>GSHMASMTGGQQMGRGSMKFSFELAVNTKKEDAWTYYSQVNQWFVWEGDLEQISLEGEFTTGQKGKMKMEDMPELAFTLVEVRENQCFSDLTATPFGNVLFEHEILENPDGTISLRHSVSLTDSDTTEEALAFLKQIFADVPESVGKLKQILETV[2x]

One such case is SMU.440 (GeneID: 1029579), which is composed of 138 residues. SMU.440 is a hypothetical protein without any known functions or protein family classification. The crystal structure reveals a fold similar to known polyketide cyclases even though the amino acid sequences are quite different. SMU.440 also shares a similar binding pocket composed primarily of residues with aromatic and acidic side-chains, which points to a potential binding of a polyketide-like molecule.

The crystal structure of SMU.440 has been determined at 2.4 Å resolution using the SIRAS (single isomorphous replacement with anomalous scattering) method and all residues except the last one could be fitted into the electron density. In addition, five residues from the N-terminal His6-tag were also observed in the structure. SMU.440 is comprised of three α-helices and a seven-stranded antiparallel β-sheet, bending into an unclosed β-barrel. The structure belongs to the SCOP superfamily of Bet v1-like proteins. There are two molecules per asymmetric unit (ASU) and they form a homodimer via a pair of antiparallel β-strands. Prediction of assemblies by the PISA server indicates that this dimer interface is the largest (interface area 946.6 Å2) with a favorable interaction energy (ΔiG −6.9 kcal/mol), in agreement with the dimer state in solution observed during the gel filtration chromatography experiment. A large forked cavity is formed as the β-barrel wraps around the long C-terminal α3-helix. The volume of the cavity is about 1 050 Å3 with a surface area of ∼700 Å2. The cavity is comprised of Trp26, Trp29, Glu30, Asp32, Met50, Met52, Met55, Phe60, Phe71, Asp73, Thr75, Thr77, Val82, Phe84, His86, His100, Val102, Phe116, Ile120, Asp123, Val124 and Ser127, most of which are quite conserved residues among the SMU.440 homologs. In the bottom of the pocket are primarily aromatic residues; whereas at the top of the pocket, close to the cavity opening, the residues can be divided into two parts, one side with mainly acidic and the other with neutral residues.>PRHVRIKNWGSGMTFQDTLHHKAKGILTCRSKSCLGSIMTPKSLTRGPRDKPTPPDELLPQAIEFVNQYYGSFKEAKIEEHLARVEAVTKEIETTGTYQLTGDELIFATKQAWRNAPRCIGRIQWSNLQVFDARSCSTAREMFEHICRHVRYSTNNGNIRSAITVFPQRSDGKHDFRVWNAQLIRYAGYQMPDGSIRGDPANVEFTQLCIDLGWKPKYGRFDVVPLVLQANGRDPELFEIPPDLVLEVAMEHPKYEWFRELELKWYALPAVANMLLEVGGLEFPGCPFNGWYMGTEIGVRDFCDVQRYNILEEVGRRMGLETHKL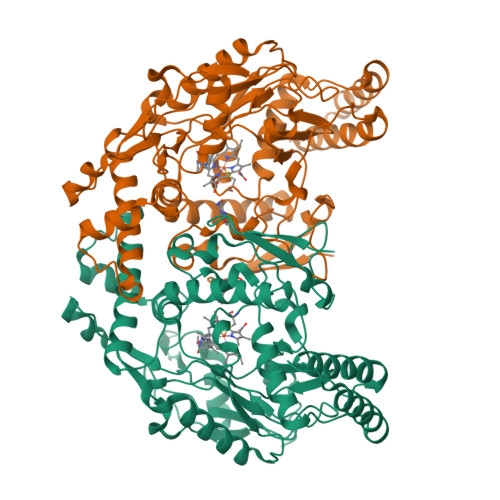ASLWKDQAVVEINIAVLHSFQKQNVTIMDHHSAAESFMKYMQNEYRSRGGCPADWIWLVPPMSGSITPVFHQEMLNYVLSPFYYYQVEAWKTHVWQDEK[4x]> SSVVVDTNGQPVSNGADAYYLVPVSHGHAGLALAKIGNEAEPRAVVLDPHHRPGLPVRFESPLRIN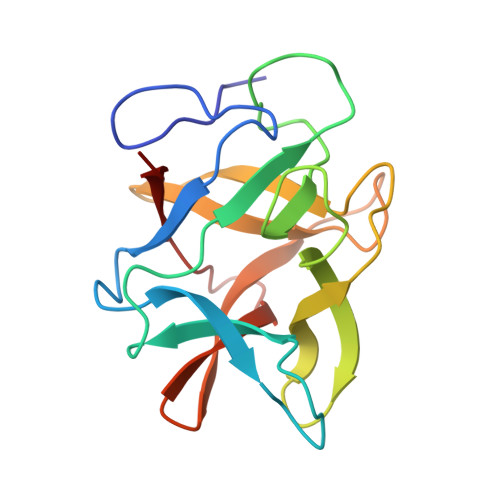IIKESYFLNIKFGPSSSDSGVWDVIQQDPIGLAVKVTDTKSLLGPFKVEKEGEGYKIVYYPERGQTGLDIGLVHRNDKYYLAVKDGEPCVFKIRKAT>MDAFQGILKFFLNQKTVIGYSFMALLTVGSERLFSVVAFKCPCSTENMTYGLVFLFAPAWVLLILGFFLNNRSWRLFTGCCVNPRKIFPRGHSCRFFYVLGQITLSSLVAPVMWLSVALLNGTFYECAMSGTRSSGLLELICKGKPKECWEELHKVSCGKTSMLPTVNEELKLSLQAQSQILGWCLICSASFFSLLTTCYARCRSKVSYLQLSFWKTYAQKEKEQLENTFLDYANKLSERNLKCFFENKRPDPFPMPTFAAWEAASELHSFHQSQQHYSTLHRVVDNG[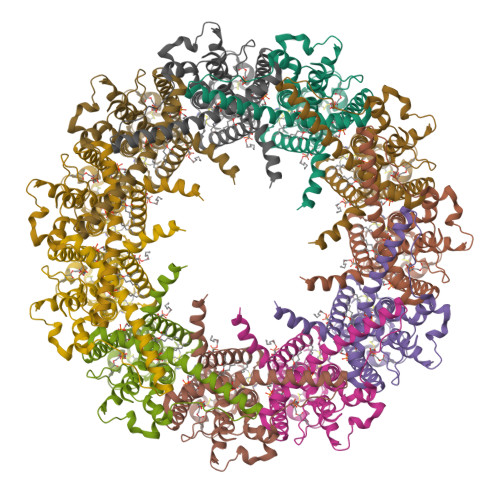11x]> MSVEGLGKDFCGAIIPDNFFPIEKLRNYTQMGLIRDFAKGSAVIMPGEEITSMIFLVEGKIKLDIIFEDGSEKLLYYAGGNSLIGKLYPTGNNIYATAMEPTRTCWFSEKSLRTVFRTDEDMIFEIFKNYLTKVAYYARQVAEMNTYNPTIRILRLFYELCSSQGKRVGDTYEITMPLSQKSIGEITGVHHVTVSRVLASLKRENILDKKKNKIIVYNLGELKHLSEQTSYYSDPNSSSVDK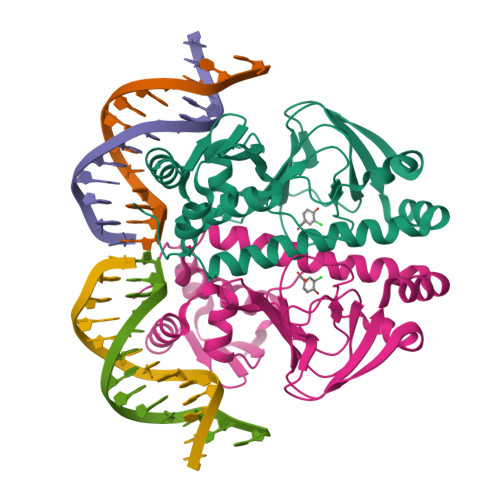LAAALDHH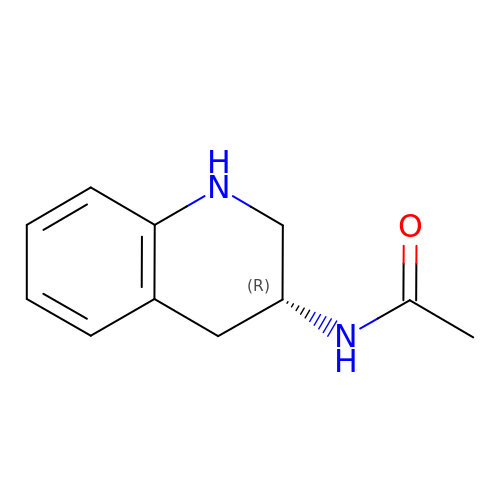~{N}-[(3~{R})-1,2,3,4-tetrahydroquinolin-3-yl]ethanamide | C11 H14 N2 O | HCEIEGOMGWEGOJ-SNVBAGLBSA-N N-(2,3-dihydroxybenzoyl)-4-(4-nitrophenyl)-L-threonine 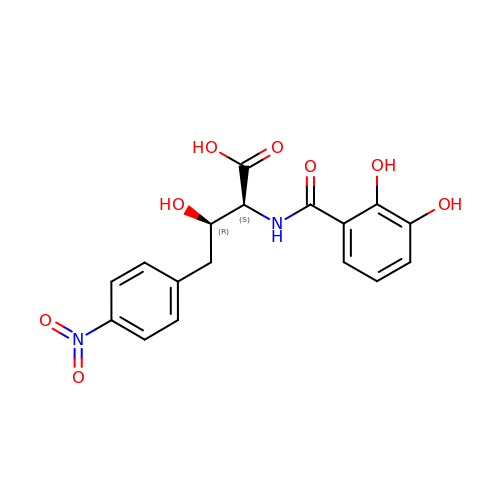| C17 H16 N2 O8 | IKEPVTXZQSIGBO-KGLIPLIRSA-N> MESXXXXXXXXXXXXXXXXXXXXXAKLLWLPLPMLMMLIVATVGVLVAVWLERKISAAVQQRIGPEYIGPLGILAPLADGLKLIFKEDVLPANSDRWLFTLGPAVVVIPVFLSYIIVPFGQNLLISNLAMGVFLWIALSSIAPIGLLMAGYASNNKYSLLGGLRAAAQSISYEIPLALAVLAVAMMSNGLGTVEIVEQQSQYGILSWNVWRQPIGFLVFWIAALAECERLPFDLPEAEEELVAGYQTEYAGMKFALFYLGAYVNLVLSALLVSVLYFGGWSFPIPLETIANLLGVSETNPFLQIAFAVLGITMTLIKAYFFVFLAILLRWTVPRVRIDQLLDLGWKFLLPVGLVNLLLTAGLKLAFPVAFGG;> MDLVTLAGQLNAGTILPETILIVTLLVVLLADLIQGRQADRWTPYFAIVGLGGAIATMIPLWTQPATISFFGSFISDHLSLFFRGLIALSALGTILMSIRYVEQTGSSLGEFMTILLTATVGGMFIAGAQELVFIFVALETLSIASYLLTGYTKRDSRSNEAALKYLLIGAASSAIFLYGSSLLYGLSGGHTQLPAIAQALSSESLGLVVALVFVIAGISFKISAVPFHQWTPDVYEGAPTPVVAFLSVGSKAAGFALAIRFLTLAFPSVTDQWQLIFTVLAILSMILGNVVALAQTSMKRMLAYSSIGQAGFVMIGFVVGTEAGYASMLFYLLVYLFMNLGAFTCVILFSLRTGTDQISEYAGLYQKDPLLTLGLSLCLLSLGGIPPLAGFFGKIYLFWAGWQAGAYGLVLLGLLTSVISIYYYIRVVKMMVVKEPQEMSEAVRNYPEVSWSSFGLRPLQVGLVMTVIATSLAGILANPLFNLVNTAVWDVPQLANQPTVMEVAYQALSPAGKS;> MVAIPRLRDTATVFVLSGYEYFLGFLIICSLVPVLALAASALLRPKSGRMIRLTTYESGMEPIGGAWIQFNVRYYMFALVFVIFDVETVFLYPWAVAFHQLGLLAFIEALIFIAILVVALVYAWRKRALEWS;> MSTFPWLTTIILFPIVAALAIPFIPDPTGKGRPIRWYALAVGLIDFALIVYAFTNFYDLNTPGMQLWESYDWIPEIGLRWSVGADGLSMPLILLTGFITTLAILAAWPVTLKPRLFYFLMLAMYGGQIAVFAVQDMLVFFLAWELELIPVYLLLAIWGGHKRQYAATKFILYTAGSSLFILVAGLAMAFYGDTVSFDMQTLAAKDYALGFQLLVYAGFLVAYGVKLPIVPLHTWLPDAHGEATAPVHMLLAGILLKMGGYALIRMNVDMLPAAHAKFAPVLVILGVVNIIYAALTSYAQRNLKRKIAYSSISHIGFVLIGIASFTNLGMSGAVLQMVSHGLIGASLFFLVGATYDRTHTLILEEMGGVGQKMKKIFAMFTACSLASLALPGMSGFVAELMVFIGFATSDAYSLPFRVIVVFLAAVGVILTPIYLLSMLREIFYGPENKELVEHEALVDAEPREVFIIACLLVPIIGIGLYPKLLTQIYDATTGQVIARAREVLPTLAQQTEQPLGILPMVAPQLKANAQ;> MQLTYVLILAALLFCIGIYGLVTSRNAVRVLMSIELLLNAVNLNLIGFANYLDGQQIKGQVFAVFVITVAAAEAAVGLAIILAIYRNRDTVDMEKFNLLKW;> MEPLYQYAWLIPVLPLLGALIVGFGLIAFSETTSKLRRPSAIFIMALMAIAMGHSLTLFWSQVQGHLPYTQMIEWAAAGNLHIAMGYVIDPLAALMLVIVTTVAFLVMLYSDGYMAHDPGYVRFFAYLSLFGSSMLGLVVSPNLVQVYIFWELVGMCSYLLIGFWYDRKSAAEAAQKAFVTNRVGDFGLLLGMVGLFWATGTFDFAGMGDRLTELVNTGLLSPSLAAILAILVFLGPVAKSAQFPLHVWLPDAMEGPTPISALIHAATMVAAGVFLIARMFPVFEQLPQVMTTIAWTGAFTAFMGATIAITQNDIKKSLAYSTISQLGYMVMGMGVGAYSAGLFHLMTHAYFKAMLFLGSGSVIHSMEGVVGHNPDLAQDMRYMGGLRKYMPITGATFLVGCLAISGVPPFAGFWSKDEILGAVFHANPAMWLLTWLTAGLTAFYMFRMYFMTFEGKFRNVPPERQEHHDHHSHHAAVPHESPWTMTLPLVVLAIPSTLIGFVGTPFNNLFEVFIHAPGEEKVAEHAVDLTEFLILGGSSVGIGLMGITVAYLMYLKGTPSPQAIAKAIQPLYQFSLHKWYFDELYEAVFIKGCRRLARQVLEVDYNVVDGVVNLTGFVTMVTGEGLKYLQNGRAQFYALIVLLAVLGFVIFSVQT;> MDLATLTQTITFFALAAAVIIAALGVVLLDNVVYSAFLLGGVFLSIAGLYILMNADFVSAAQILIYVGAVNVLILFAIMLVNKRETYTPVPGRWLRQGGAAVVSLGVFALLTKMILQTPWQLSSVPPTPDSITTIGQHFFSDFLLPFELASVLLLMALIGAVVLARRELVLEPEPILGEEVVPPLELPERPREPVALSEK;> MPKIETRTEPMVINMGPHHPSMHGVLRLMVTLDGEDVIDCEPVIGYLHRGMEKIAENRTNIMFIPYVSRWDYAAGMFNEAVTVNAPEKLAGIPVPKRASYIRVIMLELNRIANHLLWLGPFLADVGAQTPFFYIFREREYIYDLFEAATGMRFINNNYFRIGGVAADLTYGWVTKCRDFCDYFLPKVDEYERLITNNPIFVRRLQGVGKISREEAINWGLSGPMLRASGVKWDLRKVDHYECYDDFDWDVPVATEGDCLARYIVRIQEMRESVKIIRQALDGLPGGPYENLEAKRMLEGAKSEWNGFDYQYIGKKLSPTFKIPKGEHYVRVESGKGELGIYLIGDDNVFPWRWKIRPPDFNNLQVLPQLLKGMKVADIVAILGSIDVIMGSVDR;> MKFLNQITNYAKEAVQSAKYIGQGLSVTFDHMRRRPITVQYPYEKLIPSERFRGRIHFEFDKCIACEVCVRVCPINLPVVDWVFNKELKKKELKHYSIDFGVCIFCANCVEYCPTNCLSVTEEYELATYDRHELNYDSVAMGRIPYKVTQDPMVTPIREFAYLPAGVMSGHDLPAGAQRAGERPEAIANTAKSSEN;> MSDTPEAPIVEAGPVGRLLQSQNLSVESLGRDASGVEMIKVDRDRLL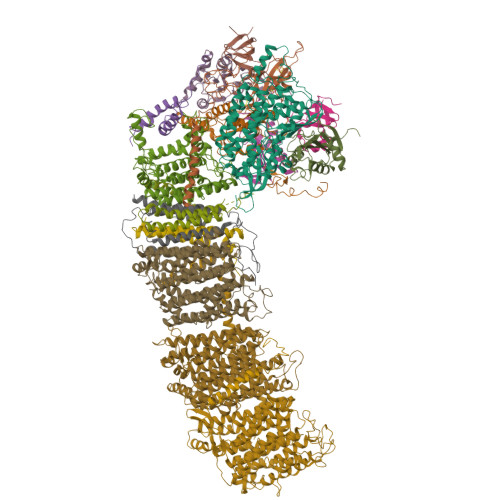AVCQTLYADGFNYLRCQAAYDSGPGQDLVSTYHLIKLSDNADRPPEVRIKVFVPRDDPRVPSVYWIWKTADWQERESYDMFGIVYEGHPNLKRILMPEDWVGWPLRKDYITPDFYELQEAY;> MTNTTSPAILNPIARPEVPQELAENIILTSLNDVYDWARLSSLWPLMYGTACCFIEFAAMIGSRFDFDRFGLVPRNSPRQADLIITSGTITMKMAPALVRLYEQMPSPKYVIAMGACTITGGMFSSDSYSAVRGVDKLIPVDVYLPGCPPRPEAIMDAIVKLRKKIANEHINERGNLAQTHRLFTAKHKMKPVPPILTGQYLNAPSRQAPPPALAAAMGIAVPALGEAVSETTSVAE;> MAVSTELLVLGVYGALAGLYLLVVPAIVYAYLNARWYVASSFERAFMYFLVTFFFPGLLLLAPFINFRPQPRSLNS;> MLLKSTTRHVHIYAGHVVDGEVHPDTETLTLNVDPDNELEWNEAALAKVEAKFRELVANAAGEDLTEYNLRRIGSDLEHFIRSLLMQGEIGYNLNSRVRNYSLGIPRVNHS;> MGLLAGYQFVKDLESAGALALFVPPEGGFEGRYQRRLRSKGYTTLPMSAPGLGDLAAYLTQEHGIRPAHTGKEDIRVYFQPPLVTYHLENLPPNAKGLVLWLIDGKRLSKQEFAYLAQLTQTLPKFKVVVEVGGDRVVRWEPLADWVAAA;> MAIKKGDLVKVVAEKLANSLEALASDHRYPPYLFEGRGEVVDIRGDYAQIKFPVPTPTVWLRLDQLEVAQ;> MDAVISVKPILLAMTPVFILLCLFFGTRNGFYDTDQYHGNGSAH;> MIRPIADTYPLLPLSKAQMGQRQEIINSHKRLWDKTMATDLIMTILPGMTVKVTNPNDTYYQFQGIVQRITDGKVAVLFEGGNWDKLVTFQASELEPVVVTPKEKAKAKK> SSIYAEDVYQNFEELKNNEDPSDYGVVTKETGSPVLVLAIHGGGIEGGTSEVARELSKEYSMYLFEGLKSAGNSVLHITSTHFDEPRALKMTGNHEYVISLHGYAEEDQQIEVGGTDRVRAADLVEKLQHAGFPAVLLNMDHPHAGVSPN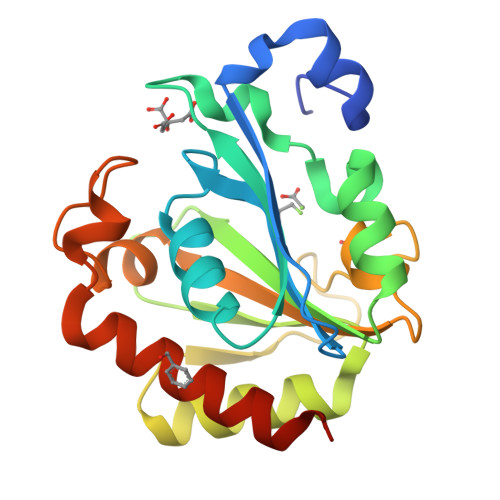NIANKSKTGLSIQIEMSTGFRKSLFGIFSLKSRAVTQNERFYEFTEVMFRFLKNSYLEHHHHHH The P pilus, produced in uropathogenic Escherichia coli, displays the adhesin PapG responsible for targeting the bacterium to the kidney epithelium. The PapA rod is formed by more than 1,000 PapA molecules assembled in a right-handed helical manner, with 3.3 molecules per turn. In a process called donor–strand complementation (DSC), the G1 β-strand of PapD inserts a conserved motif of three alternating hydrophobic residues (called the P1 to P3 residues) plus N101 (P4 residue) into four binding pockets in the hydrophobic groove of the pilus subunits (P1 to P4 binding pockets).

However, by investigating a different PapA mutant with the additional mutation T101L, we obtained crystals of a complex containing one PapD molecule and two PapANtd1_G15N_T101L molecules. This T101L mutant was initially designed to fill in the PapA P5 pocket. However, this T101L mutation had the additional unexpected consequence of stabilizing a complex containing a 1:2 molar ratio of PapD and PapA. It clearly shows one PapA molecule bound to PapD through DSC in a complex very similar to PapD/PapANtd1_G15N; however, this time, the Nte of the donor–strand-complemented PapA molecule is bound to the groove of another PapA molecule, and thus this ternary complex crystal structure provides a snapshot of PapA before and after DSE. The core sheet structure of dsePapA is in a closer conformation than that of dscPapA, as the β-strands on each side of the groove of dsePapA are nearer to each other. Also, the “63–74” loop is ordered in dsePapA and not in dscPapA, as this molecule is missing residues 70 to 73 in this region. DsePapA is only visible in the electron density from residue 20, as its Nte is not interacting in the groove of another PapA molecule and is thus disordered. Figure 3B shows the surface of dsePapA bound to the truncated Nte of dscPapA and that of dscPapA bound to the G1 strand of the chaperone: the PapD G1 strand interacts as expected at the P1 to P4 positions in the groove of dscPapA, the Nte of which interacts in the P2 to P5 pockets in the groove of dsePapA. In contrast to what is observed in the PapE/KNte or any other chaperone–subunit complex structures, the side chain of F152 has moved out of the P4 pocket of the DsePapA structure and the P4 pocket can now accommodate the N15 mutation (substituted for wild-type G15 in the PapANtd1_G15N_T101L mutant to prevent higher-order polymerization). F152 in the dsePapA structure is allowed to move away from the groove position because of the T101L mutation. Indeed, as shown in Figure 4B, the T101L mutation and the insertion of N15 induce a rearrangement of the side-chains in the P4–P5 region, leading to T99 moving out of the P5 region, thereby leaving room for F152 to substitute in its place, the new F152 position being stabilized by L101.

> AVSLDRTRAVFDGSEKSMTLDISNDNKQLPYLAQAWIENENQEKIITGPVIATPPVQRLEPGAKSMVRLSTTPDISKLPQDRESLFYFNLREIPPRSEKANVLQIALQTKIKLFYRPAAIKTRPNEVWQDQLILNKVSGGYRIENPTPYYVTVIGLGGSEKQAEEGEFETVMLSPRSEQTVKSANYNTPYLSYINDYGGRPVLSFICNGSRCSVKKEK;>APTIPQGQGKVTFNNTVVDAPCSISQKSADQSIDFGQLSKSFLEAGGVSKPMDLDIELVNCDITAFKGGNGAKKGTVKLAFTGPIVNGHSDELDTNGGTGLAIVVQGAGKNVVFDGSEGDANTLKDGENVLHYTAVVKKSSAVGAAVTEGAFSAVANFNLTYQ[2x]>[4x]MHHHHHHMAAPGGRGRSLSGLLPAQTSLEYALLDAVTQQEKDSLVYQYLQKVDGWEQDLSVPEFPEGLEWLNTEEPISVYKDLCGKIVVLDFFTYCCINCIHLLPDLHALEHTYSDKDGLLIIGVHSAKFPNEKVLDNIKSAVLRYNITHPMVNDADASLWQELEVSCWPTLVILGPRG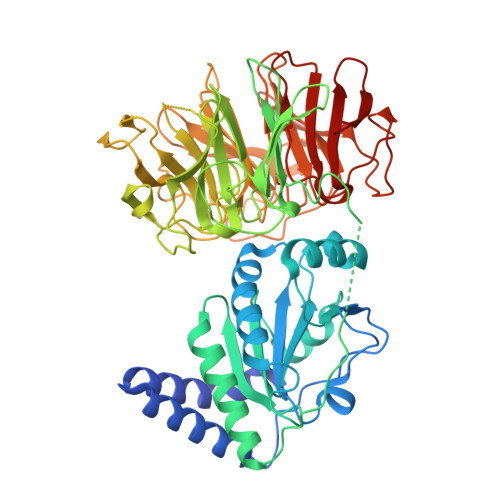NMLFSLIGEGHKDKLFLYTSIALKYYKDRGQIRDNKIGIKLYKDSLPPSPLLFPGKVTVDQVTDRLVIADTGHHRILVVWKNGQIQYSIGGPNPGRKDGIFSESTFNSPQGVAIMNNIIYVADTENHLIRKIDLEAEKVSTVAGIGIQGTDKEGGAKGEQQPISSPWDVVFGTSGSEVQRGDILWIAMAGTHQIWALLLDSGKLPKKNELTKGTCLRFAGSGNEENRNNAYPHKAGFAQPSGLSLASEDPWSCLFVADSESSTVRTVSLKDGAVKHLVGGERDPMNLFAFGDVDGVGINAKLQHPLGVTWDKKRNLLYVADSYNHKIKVVDPKTKNCTTLAGTGDTNNVTSSSFTESTFNEPGGLCIGENGELLYVADTNNHQIKVMDLETKMVSVLPIF> MSQSRDLQGGKAFGLLKAQQEERLEGINKQFLDDPKYSNDEDLPSKLEAFKVKYMEFDLNGNGDIDIMSLKRMLEKLGVPKTHLELKRLIREVSSGSEETFSYSDFLRMMLGKRSAI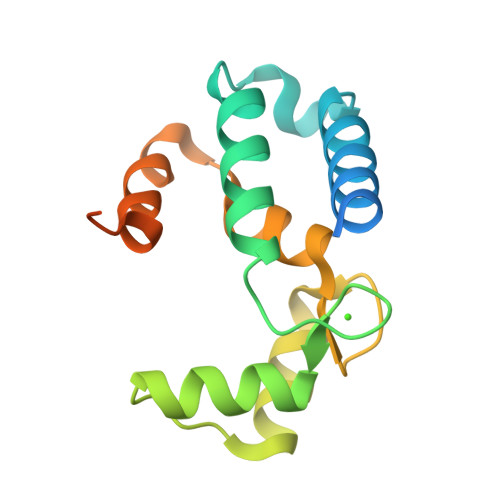LRMILMYEEKNKEHKRPTGPPAKKAISELP>GHMVSRIEQRCIDKGMKMTDQRRVIAQVLSDSADHPDVEEV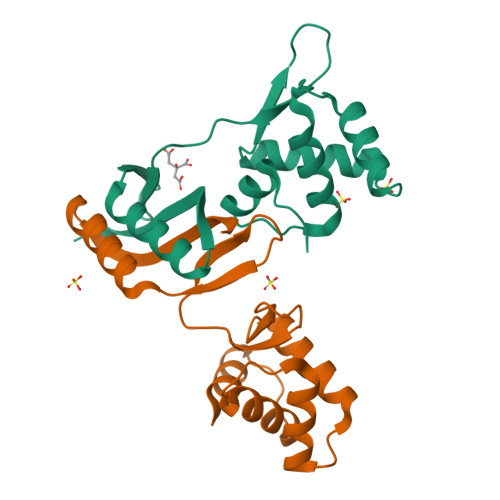YRRATAKDPRISIATVYRTVRLFEEESILERHDFGDGRARYEEAPSEHHDHLIDVNSARVIEFTSPEIEALQREIARKHGFRLVGHRLELYGVPLTSGGDSDDK[2x]>SATLKVSD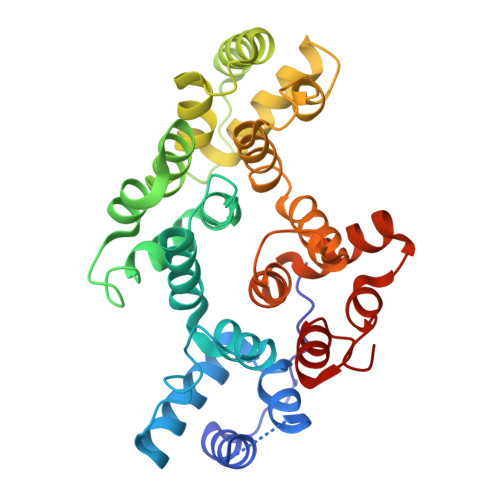SVPAPSDDAEQLRTAFEGWGTNEDLIISILAHRSAEQRKVIRQAYHETYGEDLLKTLDKELSNDFERAILLWTLEPGERDALLANEATKRWTSSNQVLMEVACTRTSTQLLHARQAYHARYKKSLEEDVAHHTTGDFRKLLVSLVTSYRYEGDEVNMTLAKQEAKLVHEKIKDKHYNDEDVIRILSTRSKAQINATFNRYQDDHGEEILKSLEEGDDDDKFLALLRSTIQCLTRPELYFVDVLRSAINKTGTDEGALTRIVTTRAEIDLKVIGEEYQRRNSIPLEKAITKDTRGDYEKMLVALLGEDDA[2x]> MGAQVSTQKTGAHETSLSASGNSIIHYTNINYYKDAASNSANRQDFTQDPSKFT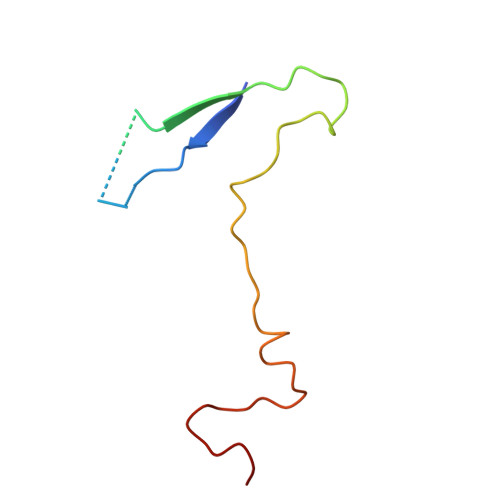EPVKDVMIKSLPALN> MRCLALDIGGTKIASAIVTDGKIEQRQQIATPQADAANAMHDTLANILALYAGQFDYVAVASTGIINHGVLTALNPKNLGGLAEFPLKESIARHTDKPIGLLNDVQAAACAEYKDEDKNAVQNFVFITVSTGVGGGIILERRLLTEPNGVAGHIGHTLADPNGPVCGCGRVGCVEAVAAGRAIEAVSSQWNPPCTPKQAFELFRKNDEKATALIQRSASAIANLIADLVIGLDVQKVVVGGSVGLAEGYLPLVKQYLNTMPHF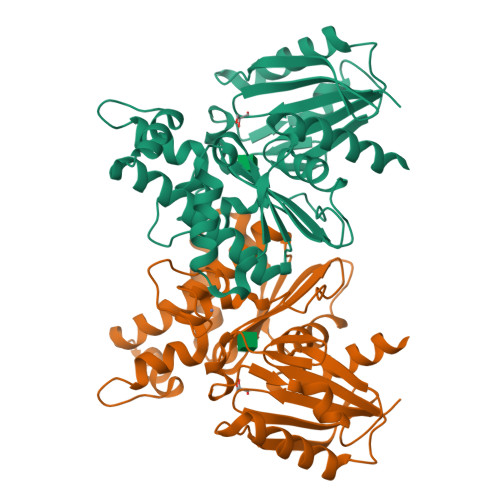YHCTVEQARHGQDAGLLGAAWWVADCLK> PQYQTWEEFSRAAEKLYLADPMKARVVLKYRHSDGNLCVKVTDDLV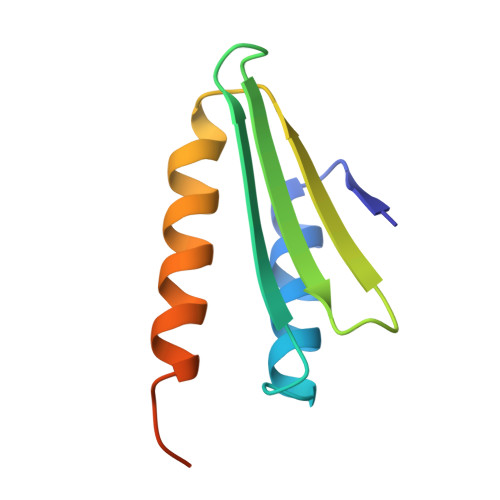SLVYKTDQAQDVKKIEKFHSQLMRLMVAKEARNVTMETE> MTTLLNPYFGEFGGMYVPQILMPALNQLEEAFVSAQKDPEFQAQFADLLKNYAGRPTALTKCQNITAGTRTTLYLKREDLLHGGAHKTNQV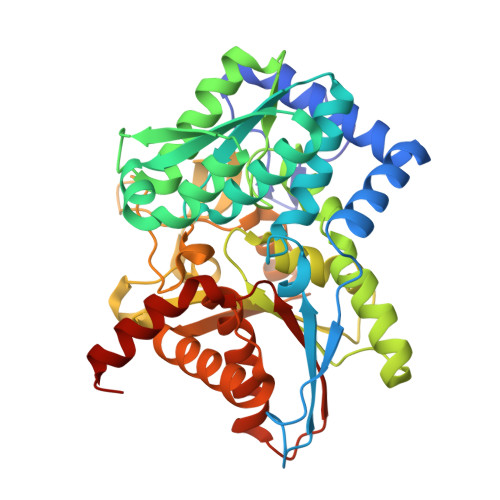LGQALLAKRMGKSEIIAETGAGAHGVASALASALLGLKCRIYMGAKDVERQSPNVFRMRLMGAEVIPVHSGSATLKDACNEALRDWSGSYETAHYMLGTAAGPHPYPTIVREFQRMIGEETKAQILDKEGRLPDAVIACVGGGSNAIGMFADFINDTSVGLIGVEPGGHGIETGEHGALLKHGRVGIYFGMKAPMMQTADGQIEESYSISAGLDFPSVGPQHAYLNSIGRADYVSITDDEALEAFKTLCRHEGIIPALESSHALAHALKMMREQPEKEQLLVVNLSGRGDKDIFTVHDILKARGEI TRAF7 serves as a crucial intracellular adaptor and E3 ubiquitin ligase involved in signal transduction pathways, contributing to immune responses, tumor progression, and embryonic development. TRAF7 is a noncanonical member of the TRAF family, with a long CC domain and distinct WD40 repeats instead of the TRAF-C domain. TRAF7 contains a RING domain, a ZF domain, a CC domain, and seven WD40 repeats. Somatic mutations within the coiled-coil (CC) domain and WD40 repeat domain of TRAF7 could cause brain tumors, while germline pathogenic mutations contribute to severe developmental abnormalities.

The structure of TRAF7 CC (fragment 270–379 aa) was solved at 3.3 Å resolution by X-ray diffraction. As predicted, TRAF7 CC forms a parallel CC trimer in the crystal, and residues E285–L377 exhibit distinct electronic cloud density and form coiled coil. Using the multi-angle light scattering (MALS) assay, we demonstrated that both TRAF7 CC and TRAF7 ZF-CC (fragment 221–379 aa) independently form trimers in solution. Detailed structural analysis revealed that TRAF7 CC comprises 10 regular heptad repeats and one hendecad repeat interspersed between the heptad repeats. The helical diagram analysis revealed that the residues at the a and d positions of the heptad/hendecad repeats of TRAF7 CC (residues in yellow in Figure 4A) are predominantly hydrophobic residues, which are mainly responsible for forming the folding core of the trimer. Charge residues in the e and g positions further stabilize the CC structure by shielding the hydrophobic core from the surrounding solution. MALS assays showed that the L322R and L347R mutants displayed significantly lower molecular weights than the wild-type TRAF7 CC. MALS assays revealed that K346E exhibited a lower molecular weight compared to the wild-type TRAF7 CC, while R371G did not present a significant difference in molecular weight, suggesting a weakened stability of the TRAF7 homotrimer caused by the K346E mutation. The results showed that the Q310L mutant behaved similar to the wild-type TRAF7 CC, while the elution peaks of the F337S and I368S variants were shifted to the right, suggesting weaker interactions between the chains of the trimer, indicating that the F337S and I368S variants likely form the trimer with lower structural stability, ultimately affecting TRAF7 function. In conclusion, our results showed that TRAF7 CC region formed a stable functional trimer in solution, and the formation and stabilization of the CC trimer are crucial for zebrafish embryonic development.

>GPGSEFELRRQGNQDTYETHLETCRFEGLKEFLQQTDDRFHEMHVALAQKDQEIAFLRSMLGKLSEKIDQLEKSLELKFDVLDENQSKLSEDLMEFRRDASMLNDELSHINARLNMGILGS[3x]>AEAGITGTWYNQLGSTFIVTAGADGALTGTFESAVGNAESRYVLTGRYDSAPATDGSGTALGWTVAWKNNYRNAHSATTWSGQYVGGAEARINTQWLLTSGTTEANAWK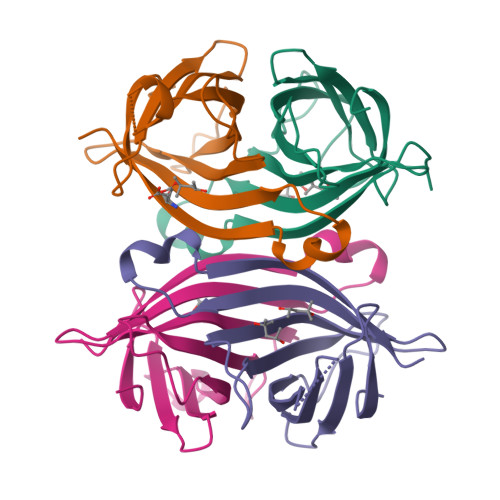STLVGHDTFTKVKPSAAS[4x]> DVQPETCRPSAASGNYFPQYPEYAIETARL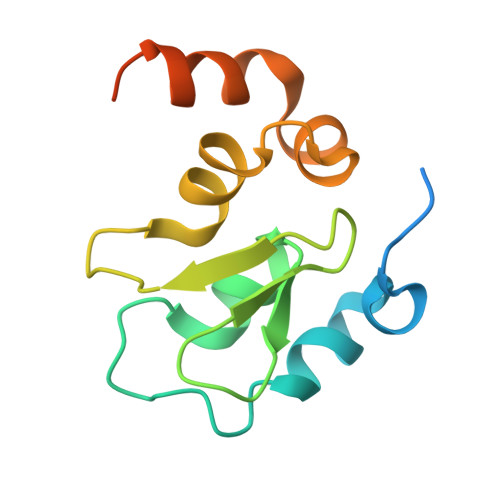RTFEAWPRNLKQKPHQLAEAGFFYTGVGDRVRCFSCGGGLMDWNDNDEPWEQHALWLSQCRFVKLMKGQLYIDTVAAKPVLAEEKEESTSIGGD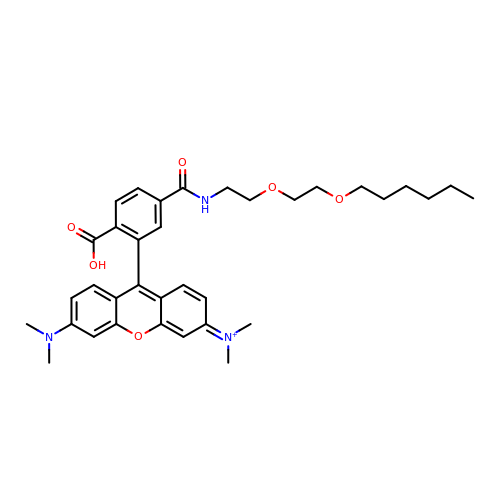9-[2-carboxy-5-({2-[2-(hexyloxy)ethoxy]ethyl}carbamoyl)phenyl]-6-(dimethylamino)-N,N-dimethyl-3H-xanthen-3-iminium | C35 H44 N3 O6 | HKVFTIWQXRNXNR-UHFFFAOYSA-O>MAQQTPLYEQHTLCGARMVDFHGWMMPLHYGSQIDEHHAVRTDAGMFDVSHMTIVDLRGSRTREFLRYLLANDVAKLTKSGKALYSGMLNASGGVIDDLIVYYFTEDFFRLVVNSATREKDLSWITQHAEPFGIEITVRDDLSMIAVQGPNAQAKAATLFNDAQRQAVEGMKPFFGVQAGDLFIATTGYTGEAGYEIALPNEKAADFWRALVEAGVKPCGLGARDTLRLEAGMNLYGQEMDETISPLAANMGWTIAWEPADRDFIGREALEVQREHGTEKLVGLVMTEKGVLRNELPVRFTDAQGNQHEGIITSGTFSPTLGYSIALARVPEGIGETAIVQIRNREMPVKVTKPVFVRNGKAVA[4x];>MSNVPAELKYSKEHEWL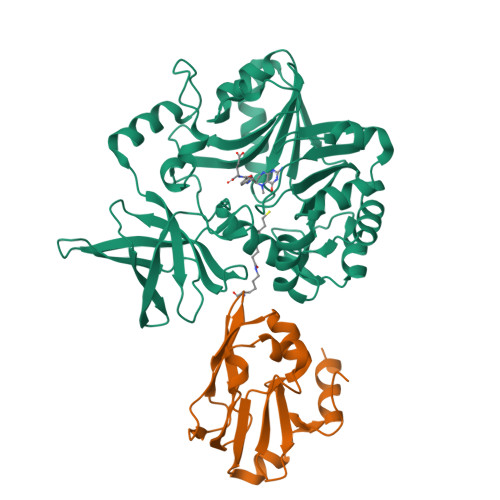RKEADGTYTVGITEHAQELLGDMVFVDLPEVGATVSAGDDCAVAESVKAASDIYAPVSGEIVAVNDALSDSPELVNSEPYAGGWIFKIKASDESELESLLDATAYEALLEDE[2x]> GSHMANPLAPYTLPQIATKVQVKHVPGKGRCLYTKHDLEPGSIIFVETPVLVAIPSLDEELWSVLTEINDEEALELPPVWHLAAICSLTMLDDEKKKICLDKWVPDPDRAPSDDVLRVINRAGLQVHPKLYERMLMVWRYNSFGHHTEQHGLVLYNRISMMAHSCRATACWHYGEDDAFILRARVKLQAGDELTISYIGDDDLFKSTNVRREKVYGWLFTCQCVRCAAPVDNARGFRCPLCGTGAMFFKTEDGETTSSACTICQAFPTQET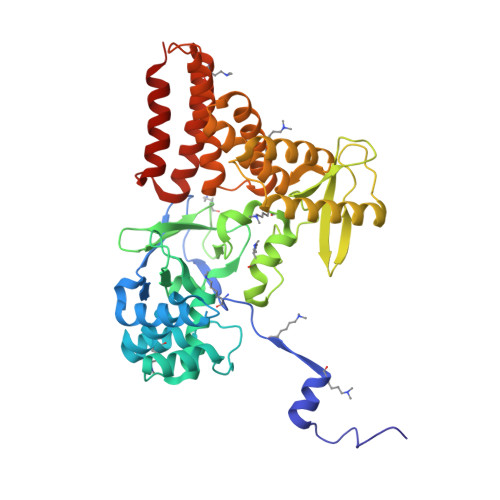IQEYLDFEQAYVDRLAETDKSDVPDAELVYNQATRVFAQHWVLYQLHTILFEGYRDAGNSESASFHQMERIKYVSQVMPLASYTLAWLYEEMGDTMLNKAEESGPEVPAHKLNVISRHFEDAYNLLYILCGEDHDYTVAAGTKKTACEERLP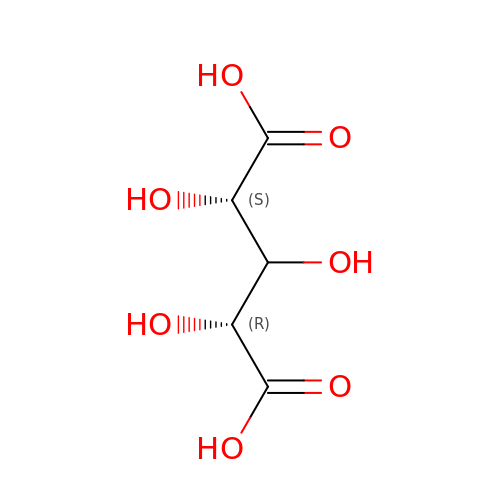D-xylaric acid | C5 H8 O7 | NPTTZSYLTYJCPR-FFEAPLRNSA-N>[4x]SEFNVKIYKLSAYGIKPNSGKNTTPLL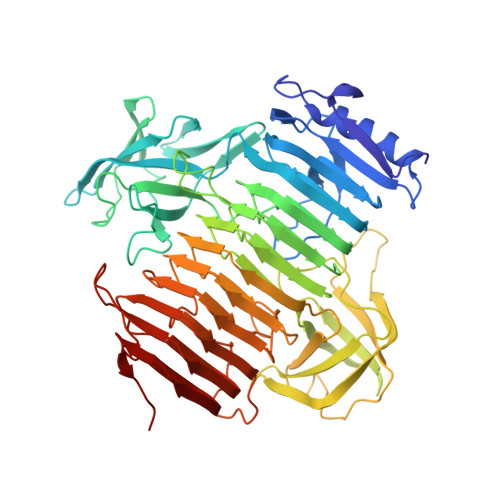TSLLKEIKSKTSDLDKVIIQFEKGRYDFYPEGAIKREYYISNHDQDNPKTVGIGIEKFNNITLIGKGTDLMFHGRMLPLALIESSNVKIKDLNIDFEKPQITQVKIISNDTTAGNIVFETAPWVKYKLKDSTFYNTGEGWEMQPTSGIAFENGTKHIIFNSGDIGVGTKSVSEVSPGKIMAHHWKNKKLVPGTVIAMRSWQRPAPGIFVHKGKNISFENVKVHYAEGMGLLAQLTENIYMDGFGVCLRGKNDPRYFTTQADATHFSGCKGEIVSKNGLYEGMMDDAINIHGTYLKITKKLDDHTVIANYMHEQSYGFDWGNIRDTVQFIQSKTMELWDAKNTIASIKPILRNSTDPIKEFRIEFTKALDPVIDPSKQDIGIENLSWTPSVVFTGNTIRNNRARGALFSTPKPTLVANNLFDHTSGCAILLCGDSNGWYETGSCRDITIRDNKFVNALTSMYQFTSAIISIYPEIPDLTNQKKYFHSGIRILNNQFDTFDQPILYAKSVDGLVFTGNKIQTNKEYPAFHSNKKRFLFERVIGVDFSDNKVDGKPIEML>MSNKCDVVVVGGGISGMAAAKLLHDSGLNVVVLEARDRVGGRTYTLRNQKVKYVDLGGSYVGPTQNRILRLAKELGLETYKVNEVERLIHHVKGKSYPFRGPFPPVWNPITYLDHNNFWRTMDDMGREIPSDAPWKAPLAEEWDNMTMKELLDKLCWTESAKQLATLFVNLCVTAETHEVSALWFLWYVKQCGGTTRIASTTNGGQERKFVGGSGQVSERIMDLLGDRVKLERPVIYIDQTRENVLVETLNHEMYEAKYVISAIPPTLGMKIHFNPPLPMMRNQMITRVPLGSVIKCIVYYKEP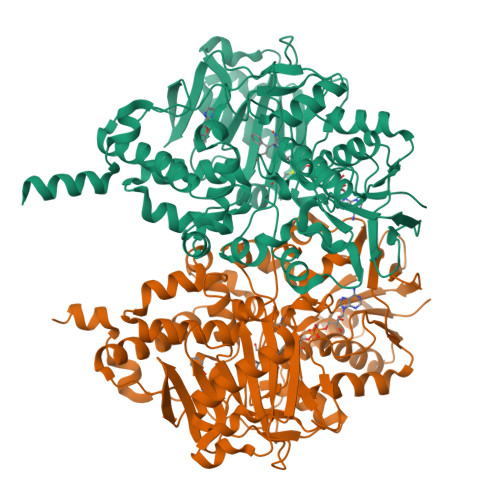FWRKKDYCGTMIIDGEEAPVAYTLDDTKPEGNYAAIMGFILAHKARKLARLTKEERLKKLCELYAKVLGSLEALEPVHYEEKNWCEEQYSGGCYTTYFPPGILTQYGRVLRQPVDRIYFAGTETATHWSGYMEGAVEAGERAAREILHAMGKIPEDEIWQSEPESVDVPAQPITTTFLERHLPSVPGLLRLIGLTTIFSATALGFLAHKRGLLVRV[2x]6-[3-(4,4-difluoropiperidin-1-yl)propyl]-4-methylpyridin-2-amine | C14 H21 F2 N3 | 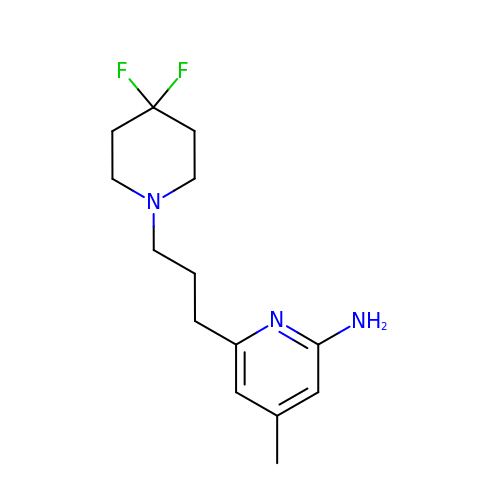QUDAAAGCJFIIKZ-UHFFFAOYSA-N> MSLTLSPLPPLSNDIYPIGR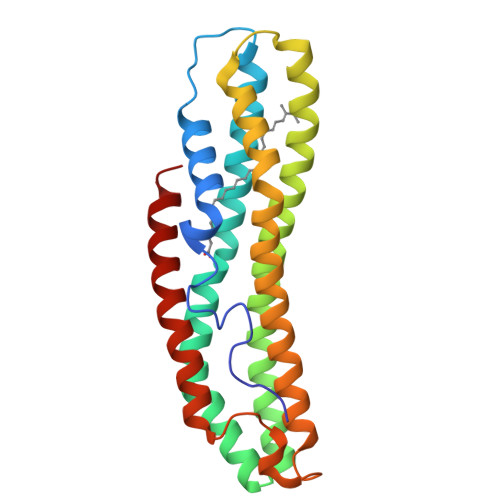NSLGNLMTATEKAKELPQEDKSAAQFQATSQESYKSAVSQTTKESPSASLAKFCKEAETAYPALYKAIQANDSASAKELAKSIASKLTEVATRAGNVAQAYNQGAAKAQEGQKLMKSALPGSHPVKDSVDDALQYLSPAAQVFTSMQSSLNESAKNVVAAADKVGKVPANQIASEDSGEAIANAWAKLGVKATAQAEAYNKWQGNQ> MSPAKEQDRFLPIANVSRIMKRSLPANAKISKE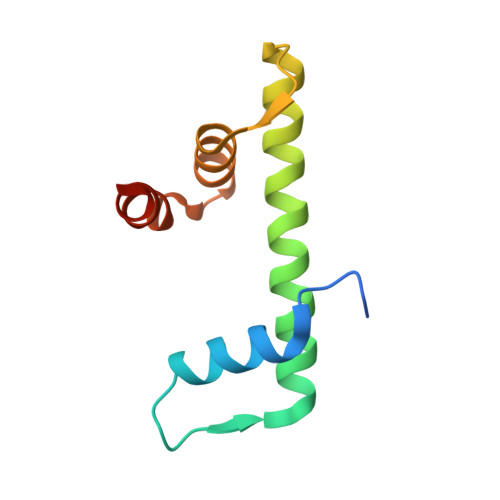AKETVQECVSEFISFVTGEASDKCQREKRKTINGDDLLWAMTTLGFEAYVGPLKSYLNRYRE>UAGCUCC[2x];>GGAGCUA[2x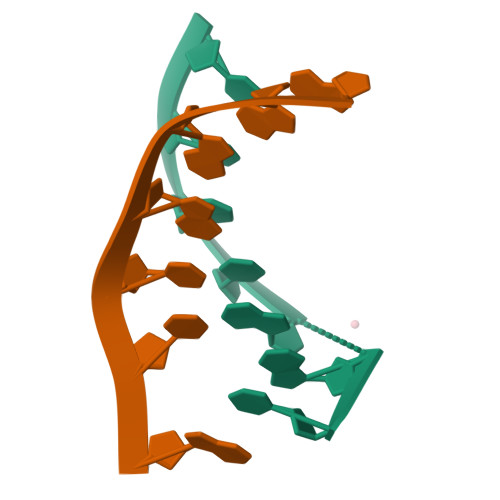]>[2x]DKIPDFVVPGKCASVDRNKLWAEQTPNRNSYAGVWYQFALTNNPYQLIEKCVRNEYSFDGKQFVIESTGIAYDGNLLKRNGKLYPNPFGEPHLSIDYENSFAAPLVILETDYSNY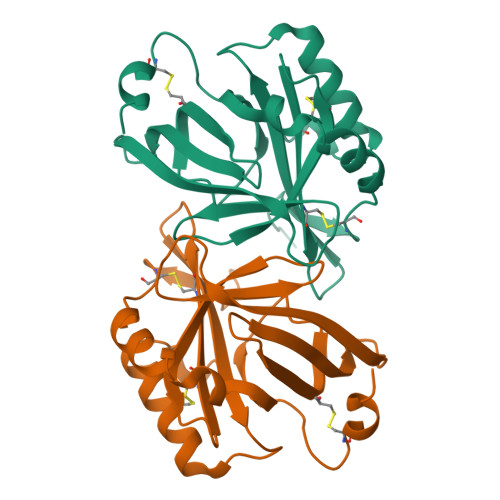ACLYSCIDYNFGYHSDFSFIFSRSANLADQYVKKCEAAFKNINVDTTRFVKTVQGSSCPYDTQKTL Recent research into cellular homeostasis has shown that the Hippo signalling pathway, which is mediated by mammalian sterile 20-like kinase (MST, the human orthologue of Hippo), controls organ size in animals and regulates cell proliferation and cell death. The MST-mediated apoptosis pathway is controlled by its interaction with RASSF family proteins and the WW45 protein. Interestingly, all three classes of tumour suppressors, MST, RASSF and WW45, interact through their SARAH (SAV/RASSF/HPO) domains. We also elucidated the MST2 homodimeric structure and performed structural and biophysical comparisons of the homodimeric and heterodimeric interactions.

Like the MST1 SARAH homodimer investigated in our previous study, the MST2 SARAH homodimer has an antiparallel helix dimer structure with a short N-terminal helix h1 folded toward h1′ of the dimeric binding partner. The main dimeric interactions consist of hydrophobic interactions of the nonpolar side chains and several inter-protomer hydrogen bonds. Firstly, the structures of the two protomers were found to be slightly different from each other in the MST2 SARAH homodimer, while those in the MST1 SARAH homodimer were identical. The distortions of the main helix h2 at the conserved proline residues in the MST2 homodimer in protomer A were 16 and 27° at Pro457 and Pro476, respectively, while those in protomer B were 12 and 15°. Thus, h2 of one protomer had a more linear structure than that of the other protomer. In addition to this difference, the hydrogen bonds between the h2 helices of the two protomers were not symmetric. When we overlaid the two protomers of the MST2 homodimer, we found that the side-chain conformations of Tyr470 and Arg474 in the two protomers differed significantly from each other, resulting in the positioning of the hydroxyphenyl group at the other side of the dimeric interface, while most of the backbone and side-chain structures converged well, with a root-mean-square deviation (r.m.s.d.) of 0.81 Å for backbone atoms and 1.22 Å for heavy atoms. The structural differences between the two protomers in the MST2 homodimer seem to arise from crystal-packing forces. In addition, the short N-terminal helices h1 and h1′ in the MST2 homodimer have been identified as typical α-helices, while those in the MST1 homodimer are 310-helices. Among the water molecules in the MST2 SARAH structure with B factor values below 25 Å2, only one water molecule mediates an inter-protomer interaction, while six water molecules in the MST1–RASSF5 SARAH structure were identified as mediators of inter-protomer hydrogen bonds.

>[2x]GSDFDFLKNLSLEELQMRLKALDPMMEREIEELRQRYTAKRQPILDAMDAK>GNSNEYRVRRERNNIAVRKSRDKAKQRNVETQQKVLELTSDNDRLRKRVEQLSRELDTLRG[2x]

pmcThe CCAAT/enhancer-binding protein (C/EBP) transcription factors belong to the basic region-leucine zipper (bZIP) family of transcription factors, which play crucial roles in tissue development, cell proliferation, and differentiation. In humans, ten C/EBP transcription factors have been identified, including six C/EBP proteins (named C/EBPα-ζ), and four C/EBP-related proteins, TEF, HLF, DBP, and NFIL3 (8, 9, 10, 11). The bZIP domain consists of a basic region (BR) and a leucine zipper region with a sequence of heptad repeats. The leucine zipper region is responsible for the dimerization of the bZIP domain, allowing the bZIP proteins to form either homodimers or heterodimers.

We then examined the DNA binding specificities of the C/EBP protein family of proteins and found that both C/EBPα and C/EBPβ also show a preference towards recognizing the TTACGTAA DNA motif. This finding was further confirmed by our structures of C/EBPα and C/EBPβ in complex with the TTACGTAA DNA. Our ITC results showed that C/EBPα and C/EBPβ bound to the TTACGTAA DNA with a Kd of ∼0.354 μM and 0.018 μM, respectively, which were 1.4- or 3.8-fold stronger than to the TTGCGCAA DNA, i.e., the reported consensus binding sequence of C/EBPα/β. To understand why C/EBPα/β prefers recognizing the TTACGTAA DNA, we determined the structures of C/EBPα and C/EBPβ in complex with the TTACGTAA DNA, respectively. Surprisingly, our binding results showed that C/EBPα bound to the TTACGTAA DNA of ∼8- to 20-fold weaker than NFIL3 and C/EBPβ. Although C/EBPα exhibited a conserved binding mode to DNA in the basic region with C/EBPβ, we found that C/EBPα carries an aspartic acid, D320, in the leucine zipper region, which is a glutamic acid in the corresponding position of the other C/EBP proteins. Structural comparison showed that the shorter side chain of D320 in C/EBPα prevented it from forming additional hydrogen bonds with N321' in the other monomer, unlike E111 in NFIL3 or E309 in C/EBPβ that formed a hydrogen bond with N112' in NFIL3 or N321' in C/EBPβ from the other monomer. Mutating D320 of C/EBPα to E enhanced its binding affinity by ∼5-fold compared to the wild-type C/EBPα.> ADNNESVIESCSNAVQGAANDELKVHYRANEFPDDPVTHCFVRCIGLELNLYDDKYGVDLQANWENLGNSDDADEEFVAKHRACLEAKNLETIEDLCERAYSAFQCLREDYEMYQNNNNAT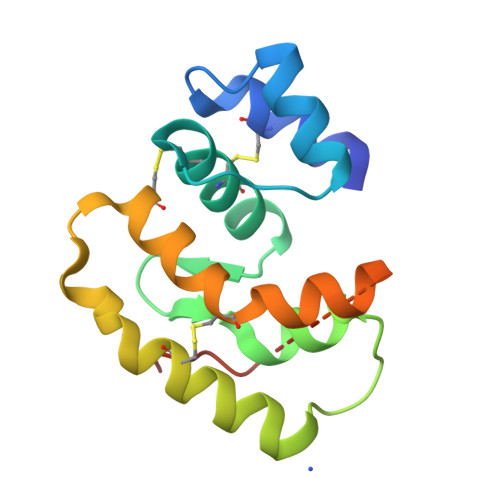SELVPRGSSGELWSHPQFEK> MALSRGLPRELAEAVAGGRVLVVGAGGIGCELLKNLVLTGFSHIDLIDLDTIDVSNLNRQFLFQKKHVGRSKAQVAKESVLQFYPKANIVAYHDSIMNPDYNVEFFRQFILVMNALDNRAARNHVNRMCLAADVPLIESGTAGYLGQVTTIKKGVTECYECHPKPTQRTFPGATIRNTPSEPIHCIVWAKYLFNQLFGEEDADQEVSPDRADPEAAWEPTEAEARARASNEDGDIKRISTKEWAKSTGYDPVKLFTKLFKDDIRYLLTMDKLWRKRKPPVPLDWAEVQSQGEETNASDQQNEPQLGLKDQQVLDVKSYARLFSKSIETLRVHLAEKGDGAELIWDKDDPSAMDFVTSAANLRMHIFSMNMKSRFDIKSMAGNIIPAIATTNAVIAGLIVLEGLKILSGKIDQCRTIFLNKQPNPRKKLLVPCALDPPNPNCYVCASKPEVTVRLNVHKVTVLTLQDKIVKEKFAMVAPDVQIEDGKGTILISSEEGETEANNHKKLSEFGIRNGSRLQADDFLQDYTLLINILHSEDLGKDVEFEVVGDAPEKVGPKQAEDAAKSITNGSDDGAQP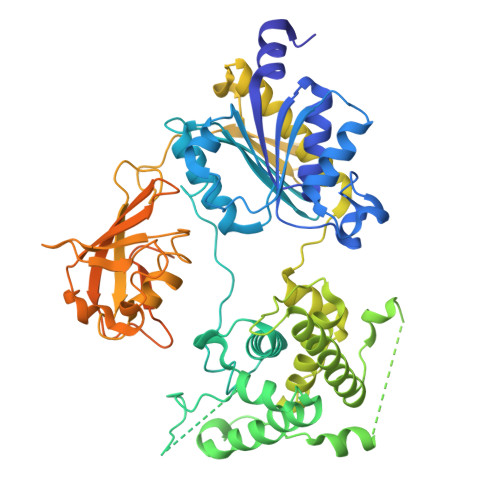STSTAQEQDDVLIVDSDEEDSSNNADVSEEERSRKRKLDEKENLSAKRSRIEQKEELDDVIALD> EGVAAALTPERLLEWQDKGIFVIQSESLKKCIQAGKSVLTLENCKQANKHMLWKWVSNHGLFNIGGSGCLGLNFSAPEQPLSLYECDSTLVSLRWRCNRKMITGPLQYSVQVAHDNTVVASRKYIHKWISYGSGGGDICEYLHKDLHTIKGNTHGMPCMFPFQYNHQWHHECTREGREDDLLWCATTSRYERDEKWGFCPDPTSAEVGCDTIWEKDLNSHICYQFNLLSSLSWSEAHSSCQMQGGTLLSITDETEENFIREHMSSKTVEVWMGLNQLDEHAGWQWSDGTPLNYLNWSPEVNFEPFVEDHCGTFSSFMPSAWRSRDCESTLPYICKKYLNHIDHEIVEKDAWKYYATHCEPGWNPYNRNCYKLQKEEKTWHEALRSCQADNSALIDITSLAEVEFLVTLLGDENASETWIGLSSNKIPVSFEWSNDSSVIFTNWHTLEPHIFPNRSQLCVSAEQSEGHWKVKNCEERLFYICKKAGHVLSDAESGCQEGWERHGGFCYKIDTVLRSFDQASSGYYCPPALVTITNRFEQAFITSLISSVVKMKDSYFWIALQDQNDTGEYTWKPVGQKPEPVQYTHWNTHQPRYSGGCVAMRGRHPLGRWEVKHCRHFKAMSLCKQPVENQEKAEYEERWPFHPCYLDWESEPGLASCFKVFHSEKVLMKRTWREAEAFCEEFGAHLASFAHIEEENFVNELLHSKFNWTEERQFWIGFNKRNPLNAGSWEWSDRTPVVSSFLDNTYFGEDARNCAVYKANKTLLPLHCGSKREWICKIPRDVKPKIPFWYQYDVPWLFYQDAEYLFHTFASEWLNFEFVCSWLHSDLLTIHSAHEQEFIHSKIKALSKYGASWWIGLQEERANDEFRWRDGTPVIYQNWDTGRERTVNNQSQRCGFISSITGLWGSEECSVSMPSICKRKKVWLIEKKKDTPKQHGTCPKGWLYFNYKCLLLNIPKDPSSWKNWTHAQHFCAEEGGTLVAIESEVEQAFITMNLFGQTTSVWIGLQNDDYETWLNGKPVVYSNWSPFDIINIPSHNTTEVQKHIPLCALLSSNPNFHFTGKWYFEDCGKEGYGFVCEKMQDTSGHGVNTSDMYPMPNTLEYGNRTYKIINANMTWYAAIKTCLMHKAQLVSITDQYHQSFLTVVLNRLGYAHWIGLFTTDNGLNFDWSDGTKSSFTFWKDEESSLLGDCVFADSNGRWHSTACESFLQGAICHVPPETRQSEHPELCSETSIPWIKFKSNCYSFSTVLDSMSFEAAHEFCKKEGSNLLTIKDEAENAFLLEELFAFGSSVQMVWLNAQFDGNNETIKWFDGTPTDQSNWGIRKPDTDYFKPHHCVALRIPEGLWQLSPCQEKKGFICKMEADIHTAEALPEKGPSHS

Most instances of MN are associated with the presence of circulating autoantibodies against a podocyte cell surface receptor, phospholipase A2 receptor (PLA2R). The PLA2R autoantibodies primarily bind to a dominant epitope located within a 31-amino acid peptide in the cysteine-rich domain (CysR) of PLA2R. PLA2R is a member of the mannose receptor family, a five-protein subgroup of the C-type lectin superfamily comprising the mannose receptor, Endo180, DEC-205, PLA2R. and FcRY. All family members contain a homologous CysR domain, fibronectin type II (FnII) domain, multiple sequential CTLDs, and a short intracellular C-terminal tail.

We expressed and purified the soluble ECD of PLA2R (residues 21–1397, spanning the N-terminal CysR to the C-terminal CTLD8 region) and performed small-angle X-ray scattering (SAXS) and cryoEM structural analysis. For single-particle cryoEM data collection, PLA2R was buffer exchanged to pH 6.2, consistent with the more compact conformation. The structure of the PLA2R ECD was determined to a resolution of 3.4 Å. The PLA2R ECD domains pack tightly together, presenting a globular structure with dimensions of ∼80 × 80 × 100 Å. Each of the tightly packed PLA2R ECDs could be built from the N-terminal CysR to CTLD8 using mostly contiguous density. It was also possible to build the initial few sugar moieties of the N-linked glycans into the cryoEM density, highlighting the dense glycosylation of PLA2R. The domain arrangements, and therefore the interdomain interactions, are different from those previously reported. The key hydrophobic residues V and I within the VIQSES sequence are located within an accessible cleft on the CysR domain, while the SVLTLENC sequence is entirely surface exposed. Of the two constituents that comprise the epitope, VIQSES occupies a surface-accessible cleft, and SVLTLENC is entirely surface exposed on the CysR domain unaffected by compaction of the structure at lower pH. Interestingly, the arrangement of the domains CysR, CTLD1, CTLD7, and CTLD8 in this structure identifies a discrete immunogenic patch on PLA2R that induces autoantibody formation and is the target for autoantibody binding.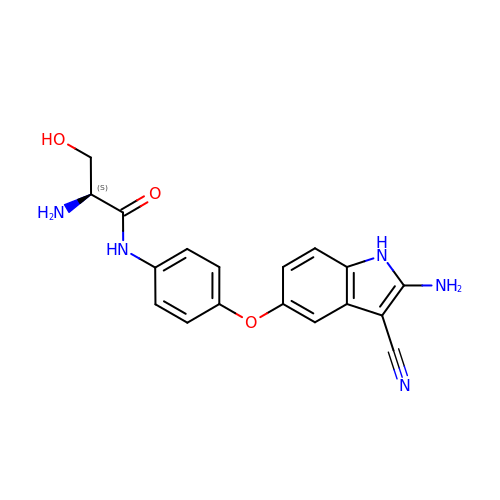(2S)-2-amino-N-[4-[(2-amino-3-cyano-1H-indol-5-yl)oxy]phenyl]-3-hydroxy-propanamide | C18 H17 N5 O3 | COLOVWUHIINYEF-HNNXBMFYSA-N>[2x]MAEGEITTFTALTEKFNLPPGNYKKPKLLYCSNGGHFLRILPDGTVDGTRDRSDQHIQLQLSAESVGEVYIKSTETGQYLAMDTDGLLYGSQTPNEECLFLERLEENHYNTYIS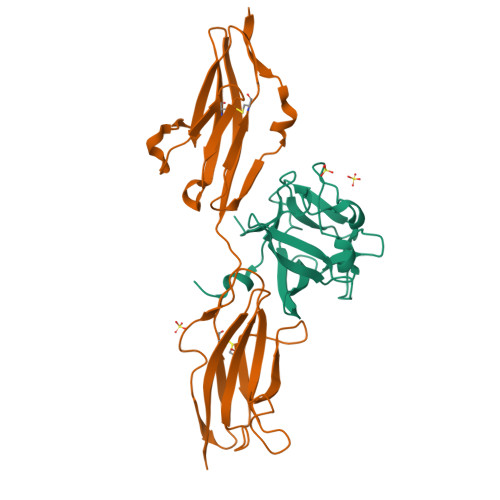KKHAEKNWFVGLKKNGSCKRGPRTHYGQKAILFLPLPVSSD;>[2x]MAEDFVSENSNNKRAPYWTNTEKMEKRLHAVPAFNTVKFRCPAGGNPMPTMRWLKNGKEFKQEHRIGGYKVRNQHWSLIMESVVPSDKGNYTCVVENEYGSINHTYHLDVVERSPHRPILQAGLPANASTVVGGDVEFVCKVYSDAQPHIQWIKHVEKNGSKYGPDGLPYLKVLKHSGINSSNAEVLALFNVTEADAGEYICKVSNYIGQANQSAWLTVLPKQQAPGREKE> SMLKRLSTEEATR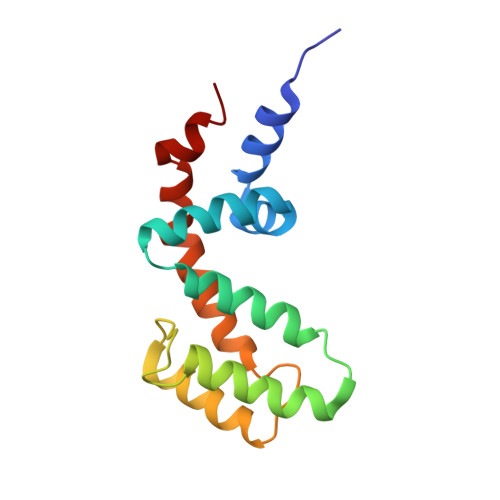WADSFDVLLSHKYGVAAFRAFLKTEFSEENLEFWLACEEFKKTRSTAKLVSKAHRIFEEFVDVQAPREVNIDFQTREATRKNLQEPSLTCFDQAQGKVHSLMEKDSYPRFLRSKMYLDLLS> MSNNNYIVPGE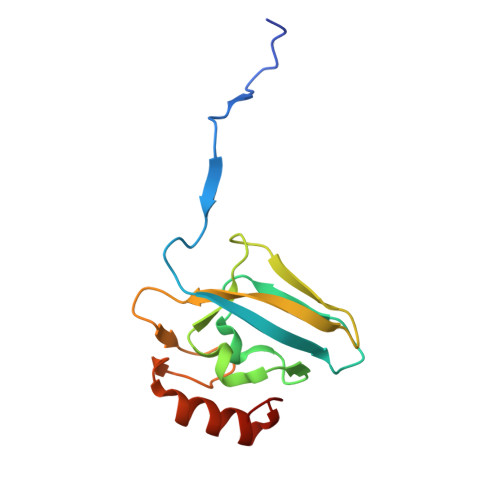YRVAEGEIEINAGREKTTIRVSNTGDRPIQVGSHIHFVEVNKELLFDRAEGIGRRLNIPSGTAARFEPGEEMEVELTELGGNREVFGISDLTNGSVDNKELILQRAKELGYKGVE>[2x]MHHHHHHENLYFQGAGAGAGAGAMTAPSALATAAAVRAGETTALAETEAAIARIEAANPDLNAVVVKDYDRARDAARALDARIAEGFDAPLLGVPMTIKESFNVAGLPTTFGVEQFRDFVAAEDAVA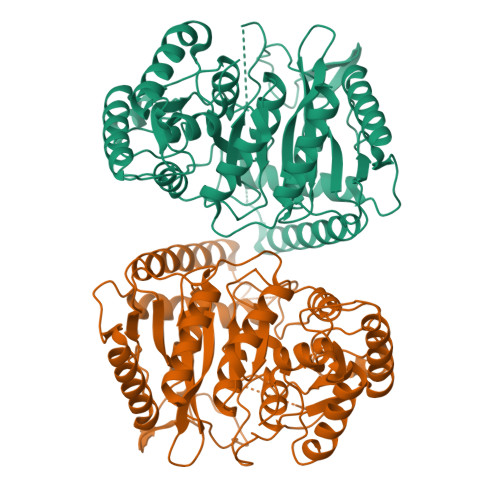VQRLKAAGTIILGKTNVPPRLADIQSNNPIYGRTRNAFDPARVAGGSSGGSAVALASGMVPLEFGSDIGGSIRVPAAFNGVWGHKPTYGVLPTDGHFFPGTDFAKSVLSVIGPLARDADDLEAALEIVADHPLAPAKRHGDQWRILLLVNAPKAKVQRAIRDAIDDLAERFRAQGATVDTASDRLPDLERQNAAYEQMLNIAMSVRGPQPPGHEPPTLATWLHLHDEQARMQRQWRRLFETYDVVIAPTVGMTAFPHDDTPLPHRRLDIDGEDTPFLHQFAFPGLATLPMLPATSVPIGRDGDGLPIGVQVIADLYQDRTALAAARAAHALAWS>MFIKPGRCPKPAVQEDFDAARYLGVWYDIQRLPNKFQKGECATATYSLSPGVGFSVFNRARLANGTIKSVIGSAIAEDPCEPAKLQFFHENAAPVPYWVLSTDYDNYALVYSCINLGASHAAYASIVSRQPTLPEETIKKLQGTMSSFGVGVDTL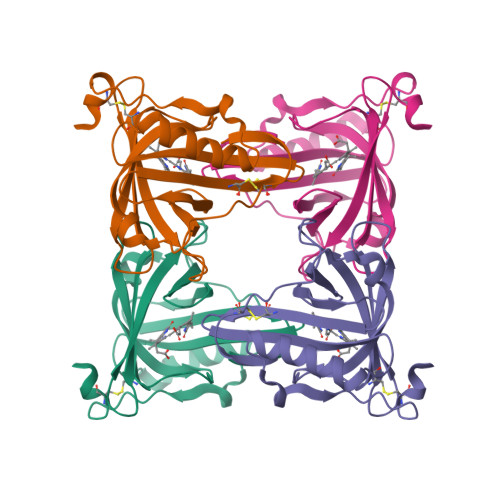LTTNQDAAYCSAMNQKLAAALEHHHHHH[2x]> GSMQRASRLKRELHMLATEPPPGITCWQDKDQMDDLRAQILGGANTPYEKGVFKLEVIIPE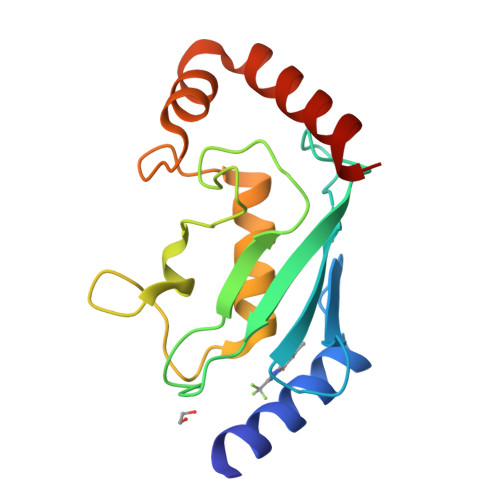RYPFEPPQIRFLTPIYHPNIDSAGRICLDVLKLPPKGAWRPSLNIATVLTSIQLLMSEPNPDDPLMADISSEFKYNKPAFLKNARQWTEKHARQK(2R)-N-hydroxy-2-methyl-2-(methylsulfonyl)-4-{2-oxo-4-[4-(2H-1,2,3-triazol-2-yl)phenyl]pyridin-1(2H)-yl}butanamide 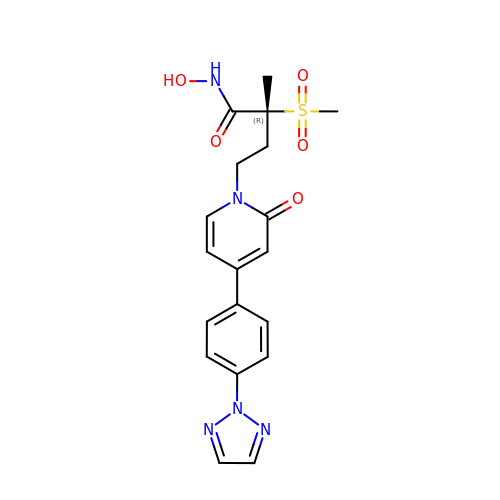| C19 H21 N5 O5 S | QSXIGYJNQBFDCD-LJQANCHMSA-N> EE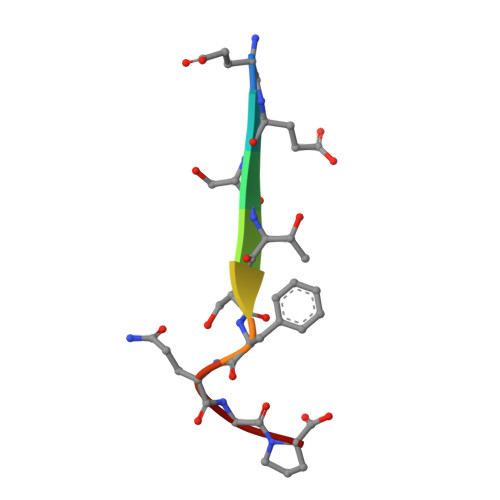STSFQGP> GAMETITVPTPIKQIFSDDAFAETIKDNLKKKSVTDAVTQNELNSIDQIIANNSDIKSVQGIQYLPNVTKLFLNGNKLTDIKPLANLKNLGWLFLDENKVKDLSSLKDLKKLKSLSLEHNGISDINGLVHLPQLESLYLGNNKITDITVLSRLTKLDTLSLEDNQISDIVPLAGLTKLQNLYLSKNHISDLRALAGLKNLDVLELFSQECLNKPINHQSNLVVPNTVKNTDG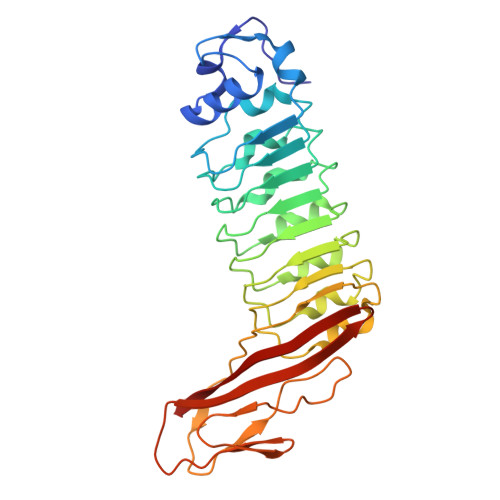SLVTPEIISDDGDYEKPNVKWHLPEFTNEVSFIFYQPVTIGKAKARFHGRVTQPLKE>[2x]ASHMFRKLAAECFGTFWLVFGGCGSAVLAAGFPALGIGFAGVALAWGLTVLTMAFAVGHISGGHFNPAVTIGLWAGGRFPAKEVVGYVIAQVVGGIVAAALLYLIASGKTGFDAAASGF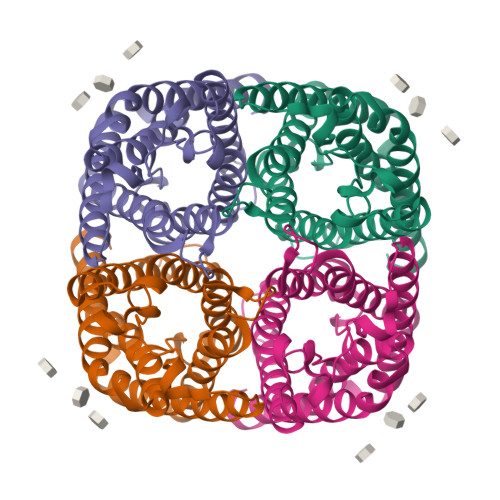ASNGYGEHSPGGYSMLSALVVELVLSAGFLLVIHGATDKFAPAGFAPIAIGLALTLIHLISIPVTNTSVNPARSTAVAIFQGGWALEQLWFFWVVPIVGGIIGGLIYRTLLEKRD> SLSSKLSVQDLDLKDKRVFIRVDFNVPLD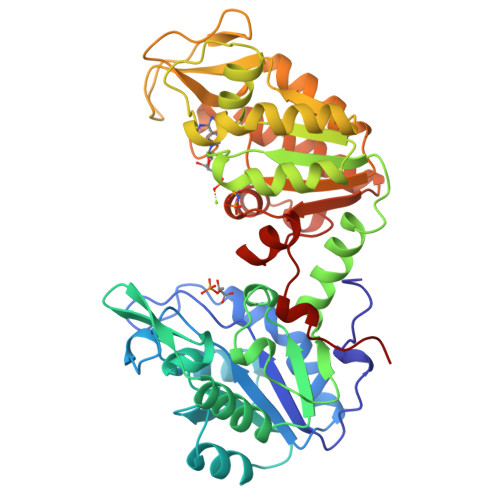GKKITSNQRIVAALPTIKYVLEHHPRYVVLASHLGQPNGERNEKYSLAPVAKELQSLLGKDVTFLNDCVGPEVEAAVKASAPGSVILLENLRYHIEEEGSRKVDGQKVKASKEDVQKFRHELSSLADVYINDAFGTAHRAHSSMVGFDLPQRAAGFLLEKELKYFGKALENPTRPFLAILGGAKVADKIQLIDNLLDKVDSIIIGGGMAFTFKKVLENTEIGDSIFDKAGAEIVPKLMEKAKAKGVEVVLPVDFIIADAFSADANTKTVTDKEGIPAGWQGLDNGPESRKLFAATVAKAKTIVWNGPPGVFEFEKFAAGTKALLDEVVKSSAAGNTVIIGGGDTATVAKKYGVTDKISHVSTGGGASLELLEGKELPGVAFLSEKK> MSYNFPAVNQLKSSKDIPDPFIFMDGSKVESTDDWWKRQSEISCMYEYYMYGKWIDGSDDETTYSISGNSMTINVKRKSTGKTASFKAVINLPKNVRHEGGAPVILGMHKGISESTATSNGYAVITYDSDGMFSAPGTAQDNNQHKGAFYDLYPYGRNWDEQTGDLMAWSWGISRILDALYNGAAKELNINPDSSIVTGVSRYGKAASVCGAFDTRIKMCAPSCSGAGGLALYRYSSVGKTYDFSSKGGSSSYTYKENEPLGSLQASGEQGWFNGRFMEFRNAEQFPMDQHMLGALCCDPDRYLFIIGSCESEDWVNAPSVWMAYLGMKHVWDYVGISDHLAINIHKSGHAVIAEDIEKMVQYFDYHVYGIQPKMNLEELQTSVFALPKNKDSFADTFASKWLYDPAFLYKVPAFLYKVVIMHHHHHH

Glucuronoyl esterases (GEs) within the carbohydrate esterase family 15 (CE15) esterase family, in a range of aerobic and anaerobic fungi and bacteria, have been identified as playing an important role in breaking down LCCs by cleaving the ester bond between 4-O-methyl-d-glucuronyl in xylan and alcohol groups in lignin. GEs share an invariant Ser-His-Glu/Asp catalytic triad and employ a conserved catalytic mechanism that involves the formation of an acyl-enzyme covalent intermediate, which is subsequently cleaved through acid-base hydrolysis. Rumen GEs adopt a canonical α/β hydrolase fold: FsCE15, PrCE15, and RfCE15 adopted the canonical α/β-hydrolase fold that is seen in all of the GE structures solved to date. The fold of all three enzymes consists of a central twisted 10 stranded mixed β-sheet flanked by α-helices on either side.

RfCE15 is the C-terminal GE domain of a multi-modular enzyme from R. flavefaciens called CesA. The structure of RfCE15 was refined to Rwork/Rfree of 16.8%/19.0% using data with a maximum resolution of 1.25 Å. The catalytic residues of RfCE15 are observed in a non-canonical configuration, with the putative general acid Glu677 located on a loop at the end of β8; making RfCE15 a member of the CE15-A GE subfamily. The general base (His714) is located on a loop directly above the catalytic serine, but is shifted by 2.2 Å relative to the position of this loop in FsCE15 and PrCE15. The shift in this position accommodates the non-canonical conformation of the general acid residue. Despite the shift in Cα of His714, the imidazole ring occupies a similar location as that found in the other GEs, with His714 Nε2 making a 2.8 Å hydrogen bond with Oγ of Ser565, and a 2.9 Å bidentate hydrogen bond with the carboxyl functional group of Glu677. Most notably, a 16 amino acid insertion from residues Gly603-Tyr619 forms an extended Ω-loop that wraps around the backside of the general base loop. As observed in other CE15-A subfamily GEs, the conserved disulfide bond found in CE15-B GEs, was not observed in RfCE15. Instead, these residues are Val564 and Val715 and form a hydrophobic pocket that is composed of an extended network of Van der Waals interactions between Ile114, Ile121, Met228, Phe314, ILE316, Ile366, and Met369. In contrast, the addition of reducing agent to RfCE15 did not alter its thermal stability, an observation consistent with the lack of disulfide bonds.5-fluoranyl-1-[4-[2-[(3~{R})-1-methyl-3-oxidanyl-2-oxidanylidene-pyrrol-3-yl]ethynyl]pyridin-2-yl]indazole-3-carboxamide | C20 H14 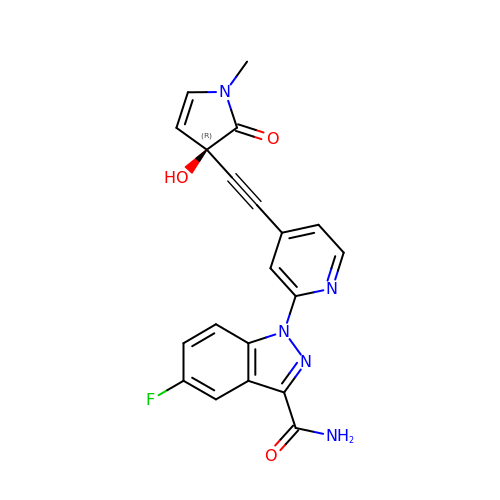F N5 O3 | ZZMZSZVGWQGKCR-FQEVSTJZSA-N3-[(4-imidazol-1-yl-6-morpholin-4-yl-1,3,5-triazin-2-yl)amino]-4-methyl-~{N}-[3-(trifluoromethyl)phenyl]benzamide | 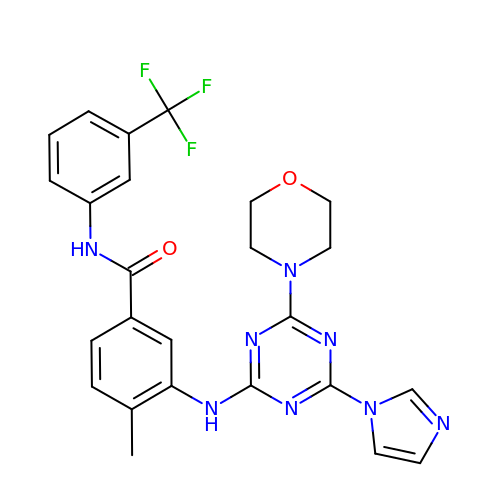C25 H23 F3 N8 O2 | AAEATOJNNUJMHY-UHFFFAOYSA-N> MDSDLKAKVESCARTADTFTRLYYASVDNRRQQIGRLYLDNATLSWNGNGAIGRQMIESYFQELPSSNHQLNTLDAQPIVDQAVSNQLAYLIMASGSVKFADQQLRKFQQTFIVTAENDKWKVVSDCYRMQE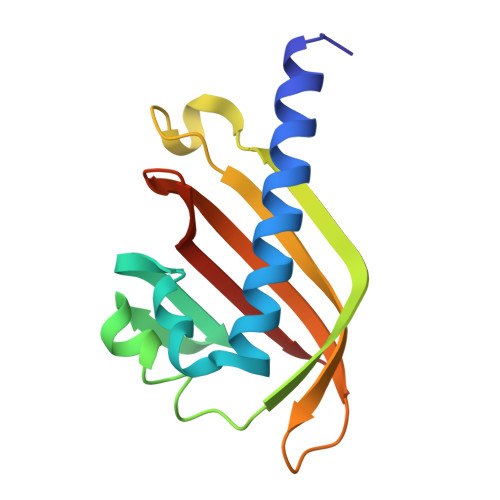V Adaptor protein complex 4 (AP-4) is part of a five-member family of heterotetrameric adaptor protein (AP) complexes, AP-1 to AP-5, known for their ability to recognize sorting signals in the cytosolic domain of transmembrane proteins destined to post-Golgi compartments. In the case of AP-4 it localizes to the trans-Golgi network (TGN;), from where it seems to participate in several sorting events, such as to the basolateral membrane in polarized epithelial cells, to the somatodendritic domain in neurons, and to early endosomes. A stronger and more functional interaction is one recently found between μ4 and a YXXØ-type, YX[FYL][FL]E motif contained in the cytosolic tail of the Alzheimer's disease amyloid precursor protein (APP). Unexpectedly, the binding site for the YX[FYL][FL]E signal of APP is located on subdomain A of the C-terminal domain of μ4, but at the opposite face of the predicted YXXØ binding site.

Surprisingly, the single mutation D190A abrogated the interaction of μ4 with the YKFFE signal. In contrast to what we expected, the single mutation D190A did not preclude the interaction of the μ4 C-terminal domain with the ENPTYKFFEQ peptide, instead the ITC analysis showed a single site on μ4-D190A with Kd = 40.6±2.6 µM. To determine whether the single D190A mutation changed the conformation of μ4, we solved the crystal structure of the C-terminal domain of μ4-D190A (residues 185–453 of the human protein) in complex with the ENPTYKFFEQ peptide from APP at 1.84 Å resolution. Similar to wild type μ4, the μ4-D190A C-terminal domain is organized into two subdomains, A and B, and has an immunoglobulin-like β-sandwich fold comprising 16 strands. The overall crystal structure is virtually identical to that of wild-type μ4, as demonstrated by a root mean square deviation of 0.190 Å for superimposable Cα coordinates. As was seen with wild type μ4, of the ENPTYKFFEQ peptide, only the TYKFFEQ portion was visible in the density map and, as expected, bound to the μ4-binding site. The area of the interface between the YKFFE signal and μ4-D190A is 431.1 Å2, analogous to that on wild type μ4 that is 430.5 Å2, as calculated by the PISA server. The μ4-D190A - YKFFE interface maintained considerable polarity, and all eight direct hydrogen bonds between μ4 and the peptide are preserved. Of all the stabilizing interactions, Y687 forms with its phenolic hydroxyl one of the shortest hydrogen bonds with the carboxylate of E265 on μ4-D190A. Additionally, Q692, the last residue in the peptide, forms a bidentate salt bridge with its free carboxylate and the guanidinium group of R283. Together, this crystallographic analysis demonstrated that μ4-D190A binds the YKFFE signal, and provided evidence against the possibility that even a minor change in conformation was the cause of the weaker interaction.

> GAMDPEFQQSKVAPSSAASRPVLSSRSDQSQKNEVFLAVVERLSVLIASNGSLLKVDVQGEIRLKSFLPSGSEMRIGLTEEFSVGKSELRGYGPGIRVDEVSFHSSVNLDEFESHRILRLQPPQGELTVMRYQLSDDLPSPLPFRLFPSVQWDRGSGRLQVYLKLRCDLLSKSQALNVRLHLPLPRGVVSLSQELSSPEQKAELAEGALRWDLPRVQGGSQLSGLFQMDVPGPPGPPSHGLSTSASPLGLGPASLSFELPRHTCSGLQVRFLRLAFRPSGNANPHKWVRHLSHSDAYVIRI;> ENPTYKFFEQ>[2x]MGQNSMDALQL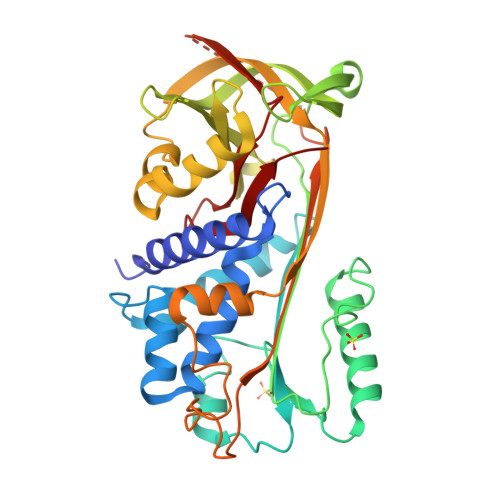ANSAFAVDLFKQLCEKEPLGNVLFSPICLSTSLSLAQVGAKGDTANEIGQVLHFENVKDVPFGFQTVTSDVNKLSSFYSLKLIKRLYVDKSLNLSTEFISSTKRPYAKELETVDFKDKLEETKGQINNSIKDLTDGHFENILADNSVNDQTKILVVNAAYFVGKWMKKFPESETKECPFRLNKTDTKPVQMMNMEATFCMGNIDSINCKIIELPFQNKHLSMFILLPKDVEDESTGLEKIEKQLNSESLSQWTNPSTMANAKVKLSIPKFKVEKMIDPKACLENLGLKHIFSEDTSDFSGMSETKGVALSNVIHKVCLEITEDGGDSIEVPGARILQHKDELNADHPFIYIIRHNKTRNIIFFGKFCSP> MRVILNTGRTIWQGQAIESGKDLKMYV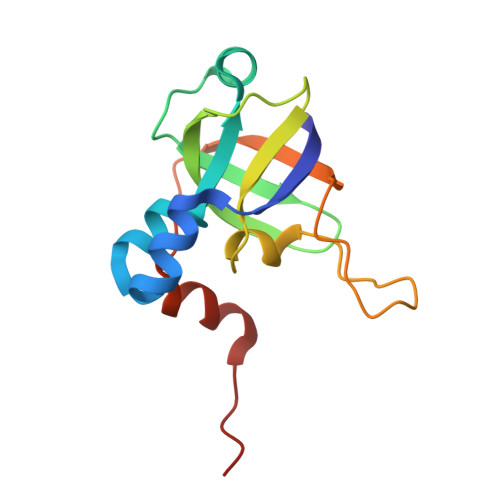DAAAIIQMNPEMMKQLGIAEGDNVKVISEYGDVVVKAVEAKEPLPEGMVYIPMGPWANRVIRPYTDSTATPSFKNIPVEIIPTDEEVLDMPTLMKVYGKVGQI> MFKLSQRSKDRLVGVHPDLVKVVHRALELTPVDFGITEGVRSLETQKKYVAEGKSKTMKSRHLHGLAVDVVAYPKDKDTWNMKYYRMIADA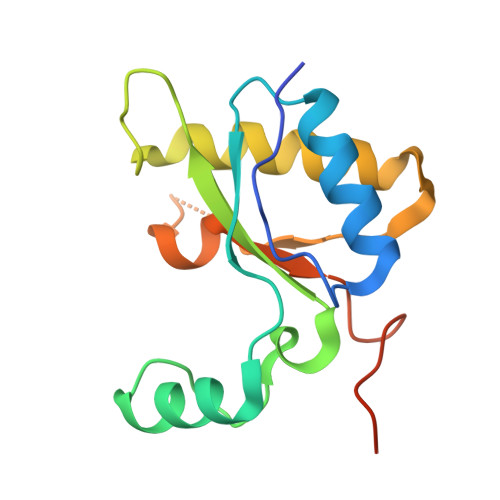FKQAGRELGVSVEWGGDWVSFKDGVHFQLPHSKYPDPKLEHHHHHHHH> ASLTEIEHLVQSVCKSYRETCQLRLEDLLRQRSNIFSREEVTGYQRKSMWEMWERCAHHLTEAIQYVVEFAKRLSGFMELCQNDQIVLLKAGAMEVVLVRMCRAYNADNRTVFFEGKYGGMELFRALGCSELISSIFDFSHSLSALHFSEDEIALYTALVLINAHRPGLQEKRKVEQL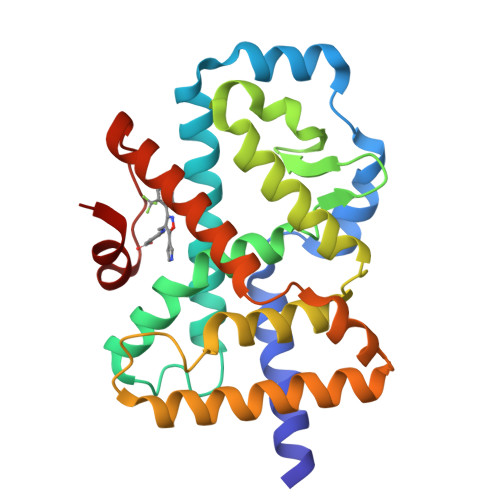QYNLELAFHHHLHKTHRQSILAKLPPKGKLRSLCSQHVERLQIFQHLHPIVVQAAFPPLYKELFS>[2x]GHMSTTARFDSIGGLFEDFTQSAAQRAIEVRTIFHMIGDVSGKSVLDLACGFGFFGREIYRRGAAKVVGVDISEKMIEL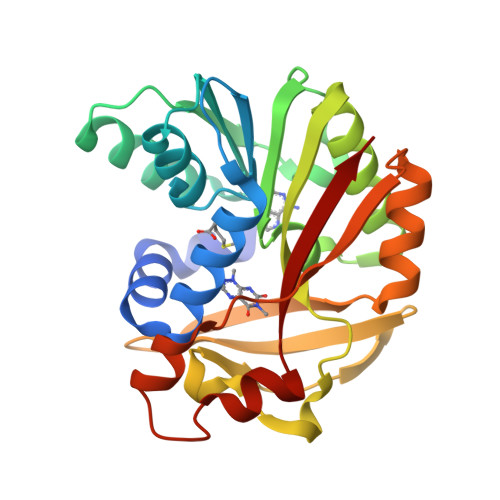AREESRKYGDPLEFHVRDVANMEPLGQFDLVNAAWLFNYADSVENLRKMFKVVRASLKPDGKLVAYTVDPDFSLAKGNFAKYGVNVLNERAWGPGYRHDAEFVTDPPSQFSFYRWSRADYESAIADAGFSHFEWQKPLLEADDIATHPPGFWDVFQNNCLQTGLVCKP> CTFCSIINRELEGYFVYEDEKFAAILDKYPVSLGHTL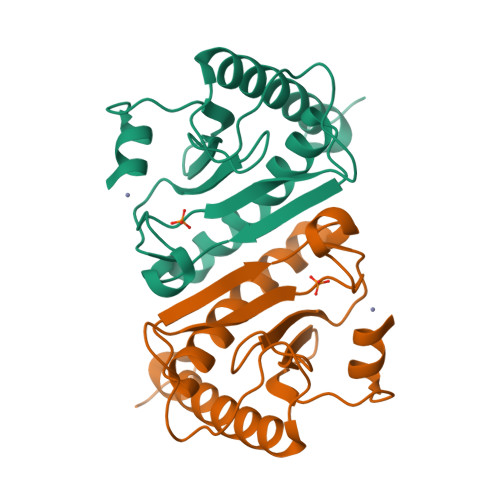VIPKKHFENYLEADEDTLAELAKVVKLVSLGIKDAVKADGLRLLTNIGRSAGQVIFHLHVHIIPTWEGDYPDIFKSFKPRKEQEKEYYELLQKIIRESIENLKRKIGDYKWG> MSLRQDILLNNNWNFRFSHQVQGDTRRVDLPHTWNAQDALAGKIDYKRGIGNYEKALYIRPEWKGKRLFLRFDGVNSIADVFINRKHIGEHRGGYGAFIFEITDLVKYGEKNSVLVRANNGEQLDIMPLVGDFNFYGGIY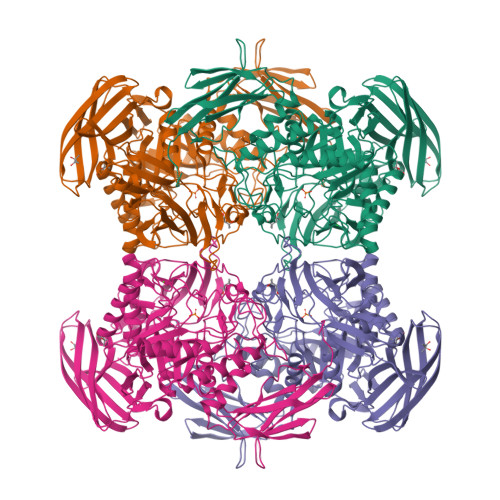RDVHLLITDETCISPLDYASPGVYLVQEVVSPQEAKVCAKVNLSNRAADGTAELQVLVTDGTKVICKESRNVSLKQGADILEQLPLLIQKPRLWNGCEDPFMYQVSISLHKDGKQIDSVTQPLGLRYYHTDPDKGFFLNGKHLPLHGVCRHQDRAEVGNALRPQHHEEDVALMREMGVNAIRLAHYPQATYMYDLMDKHGIVTWAEIPFVGPGGYADKGFVDQASFRENGKQQLIELIRQHYNHPSICFWGLFNELKEVGDNPVEYVKELNALAKQEDPTRPTTSASNQDGNLNFITENIAWNRYDGWYGSTPKTLATFLDRTHKKHPELRIGISEYGAGASIYHQQDSLKQPSASGWWHPENWQTYYHMENWKIIAERPFVWGTFVWNMFDFGAAHRTEGDRPGINDKGLVTFDRKVRKDAFYFYKANWNKQEPMIYLAEKRCRLRYQPEQTFMAFTTAPEAELFVNGVSCGKQKADTYSTVVWKNVKLTSGENIIRVTTPGKKPLTDEVTVEYKEDREGHHHHHH>MASWSHAPKFEKAGSLDSPTFGCTDSPVRRERGQKAVFCGLTSIVWLHRKMQDAFFLVVGSRTCAHLLQAAAGVMIFAEPRFGTAVLEEQDLAGLADAHKELDREVAKLLERRPDIRQLFLVGSCPSEVLKLDLDRAAERLSGLHAPHVRVYSYTGSGLDTTFTQGEDTCLAAMVPTLDTTEAAELIVVGALPDVVEDQCLSLLTQLGVGPVRMLPARRSDIEPAVGPNTRFILAQPFLGETTGALERRGAKRIAAPFPFGEEGTTLWLKAVADAYGVSAEKFEAVTAAPRARAKKAIAAHLETLTGKSLFMFPDSQLEIPLARFLARECGMKTTEIATPFLHKAIMAPDLALLPSNTALTEGQDLEAQLDRHEAINPDLTVCGLGLANPLEAKGHATKWAIELVFTPVHFYEQAGDLAGLFSRPLRRRALLNGGAA[2x];>[2x]MKLTLWTYEGPPHVGAMRVATAMKDLQLVLHGPQGDTYADLLFTMIERRNARPPVSFSTFEASHMGTDTAILLKDALAAAHARYKPQAMAVALTCTAELLQDDPNGISRALNLPVPVVPLELPSYSRKENYGADETFRALVRALAVPMERTPEVTCNLLGATALGFRHRDDVAEVTKLLATMGIKVNVCAPLGASPDDLRKLGQAHFNVLMYPETGESAARHLERACKQPFTKIVPIGVGATRDFLAEVSKITGLPVVTDESTLRQPWWSASVDSTYLTGKRVFIFGDGTHV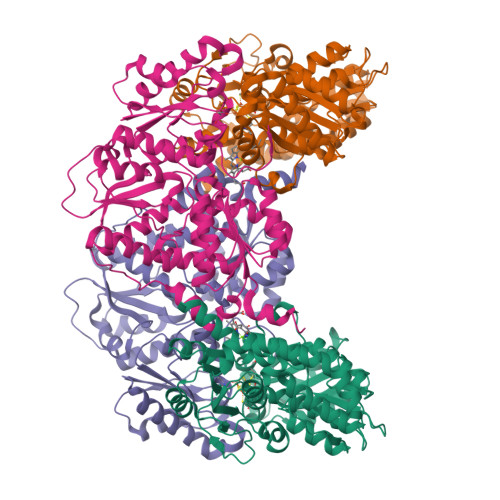IAAARIAAKEVGFEVVGMGCYNREMARPLRTAAAEYGLEALITDDYLEVEKAIEAAAPELILGTQMERNIAKKLGLPCAVISAPVHVQDFPARYAPQMGFEGANVLFDTWVHPLVMGLEEHLLTMFREDFEFHDAAGASHHGGKAVAREESPVAPADLAPAATSDTPAAPSPVVVTQASGEIRWMPEAERELRKIPFFVRGKAKRNTELYAAHKGVCDITVETLYEAKAHYAR>GSHMDYILGRYVKIARYGSGGLVGGGGKEQYVENLVLWENIIKTAYCFITPSSYTAALETANIPEKDFSNCFRFLKENFFIIPGEYNNSTENNRYSRNFLHYQSYGANPVLVQDKLKNAKVVILGCGGIGNHVSVILATSGIGEIILIDNDQIENTNLTRQVLFSEDDVGKNKTEVIKRELLKRNSEISVSEIALNINDYTDLHKVPEADIWVVSADHPFNLINWVNKYCVRANQP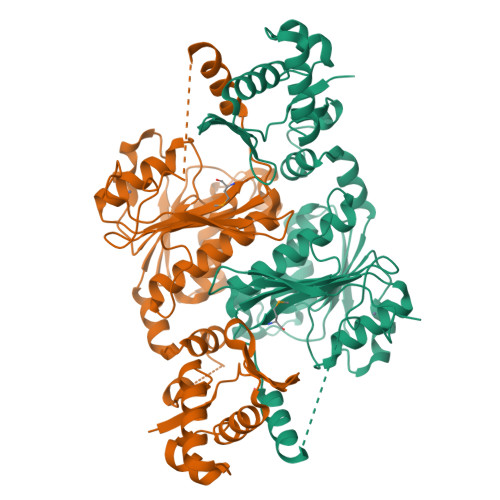YINAGYVNDIAVFGPLYVPGKTGCYECQKVVADLYGSEKENIDHKIKLINSRFKPATFAPVNNVAAALCAADVIKFIGKYSEPLSLNKRIGIWSDEIKIHSQNMGRSPVCSVCGNRM[4x];>[4x]MRTGNAN> EQTYYDLVKAFMAEIRQYIRELNLIIKVFREPFVSNSKLFSANDVENIFSRIVDIHELSVKLLGHIEDTVEMTDEGSPHPLVGSCFEDLAEELAFDPYESYARDILRPGFHDRFLSQLSKPGAALYLQSIGEGFKEAVQYVLPRLLLAPVYHCLHYFELLKQLEEKSEDQEDKECLKQAITALLNVQSGMEKICSKSLAKRRLSESACRFYSQQMKGKQLAIKKMNEIQKNIDGWEGKDIGQCCNEFIMEGTLTRVGAKHERHIFLFDGLMICCKSNHGQPRLPGASNAEYRLKEKFFMRKVQINDKDD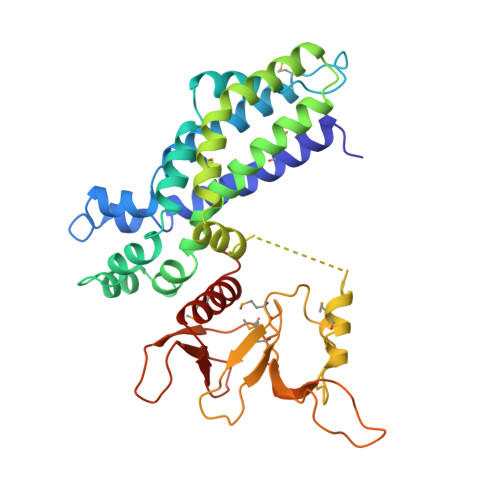TNEYKHAFEIILKDENSVIFSAKSAEEKNNWMAALISLQYRSTLE>[2x]GMSQLDKDAFEVLLANCADEPIQFPGAIQPHGLLFTLKEPELTILQVSANVQSVLGKVPDQLAGQTLDCVLGAGWAEVIRSTSANDSLVDVPRLLMSVEGVEFEALLHRSQEALVLELEIQDKAAQAISYSERTGNMGRMLRQLHAAADLQTLYEVSVREIQRMTGYDRVLIYRFEEEGHGQVIAEASAPAMELFNGLFFPASDIPEQARELYRRNWLRIIPDANYTPVPLVPQLRPDTQQQLDLSFSTLRSVSPIHCQYMKNMGVLSSMSVSLIQGGKLWGLISCGHRTPLYVSHELRSACQAIGQVLSLQISAMEALEVSRQRETKIQTLQQLHQMMATSDTDVFDGLAQQPQLLMDLVGATGVAIIEDRQTHCYGNCPEPSDIRALHTWMMAGGEPVYASHHLSSVY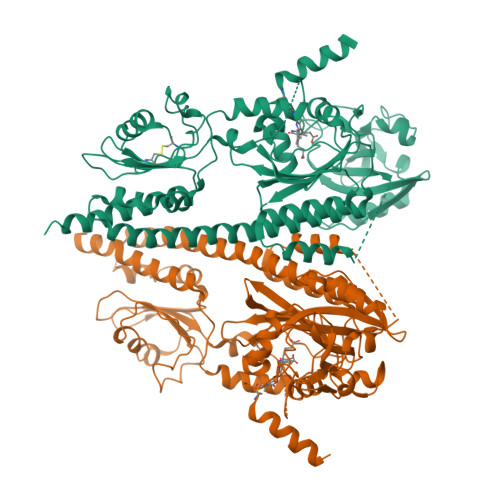PPGEAYQTLASGVLAMSLPKPVDNGVIWFRPEVKQSVQWSGDPNKPLNLDASDNTLRLQPRTSFEIWKVEMTGIATKWSHGDVFAANDLRRSALENDLARQVSKEQQAVRARDELVAVVSHDLRNPMTVISMLCGMMQKSFSSDGPHTSRRISTAIDTMQQAASRMNVLLEDLLDTSKIEAGRYTITPQPLEVSQIFEEAYTLLAPLAMDKSIEISFNAEPDIKVNADPERLFQVLSNLIGNAIKFTPKLGRIGVAAMSNGDEVVFTVRDSGEGIPPEQLPHIFERYWTVKEGNPTGTGLGLYISQGIIKAHGGELAAQSQVGHGSEFRFTVPIAH>[6x]GGTDRMARLLGELLVSTDDSGNLAVLRTPPGAAHYLA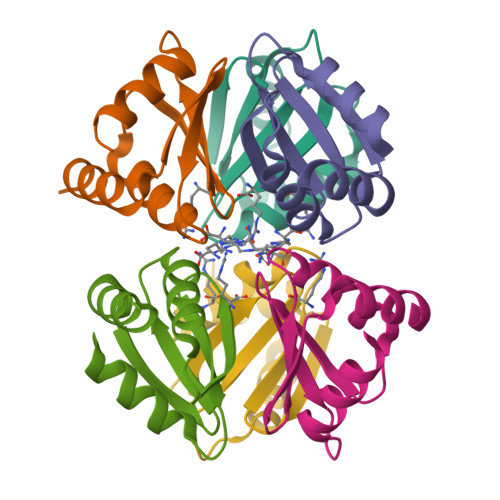SAIDRAALPQVVGTIAGDDTILVVAREPTTGAQLAGMFENLR>[2x]SNAMETTGQMPATSSLVDLLHHPLRWRITQLLIGRSLTTRELAELLPDVATTTLYRQVGILVKAGVLMVTAEHQVRGAVERT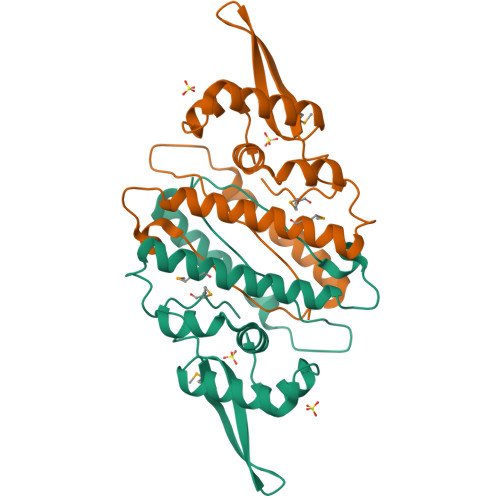YTLNTQAGDADHDGVDADRLRTMFTVFVAGVGGHLDQYLEREQIDPLADGIAFRQTALNLSDEELAEFLTAFGEFLAPYVAHSPAPDRTRRVLSTILIPD>MEISETNIGIFYVSKLLALAPYSAKKNSKGQLEITRSWLFSIYSVCLCLIMVFLTYRGLLFDANSNIPVRMKSATSKVVTASDVSVVVLAIVTGVYCGMFGLRATQELNTRLDKIDSTLSPYNNVKKDRWRAYAMATVSLIVIGILLGLDVGTWVRMAQEMNISDEDTELNVQWYIPFYSLYFILTGLHINFANTAYGLGRRYKRLNQMLRTSYLSADKSYGNATNLVKVSTVKSISFKPMMPMALHASLTKLNTETLPNESATKNKSLLIRAMADNHESLGKCVRLLSRFYGIAVLFILVSCLLHLVATAYFLFLEMLNKRDNGYVWVQMLWIIFHFLRLLMVVEPCHLAAREARKTIQIVCEIERKVFEPILVEETKKFWQQLLVDDAEFSASGLCRVNRTILTSFASAIATYLVILIQFQKTNGLEGGSSGGWSHPQFEK[4x]

While mammals use G protein-coupled receptors (GPCRs) for sweet and bitter tastant perception, insects such as fruit flies use a unique family of proteins called gustatory receptors (Grs). To unravel the overall structure of these receptors and their unique structure features that define sugar specificity, we determined the cryo-electron microscopy (cryo-EM) structures of Drosophila mojavensis Gr43a (DmoGr43a) (given its better biochemical behavior than Drosophila melanogaster Gr43a (DmGr43a)) and Drosophila melanogaster Gr64a (DmGr64a) in apo or sugar-bound states. As expected, both DmoGr43a and DmGr64a form tetramer, and are topologically similar to each other, and to Orco from Apocrypta bakeri and odorant receptor 5 from Machilis hrabei (MhOR5)11. The structures of DmoGr43a and DmGr64a can be separated into a TMD with 28 transmembranes (TMs) in total (7 TMs in each subunit, numbered as S1–S7), and an intracellular domain (ICD) containing an “anchor domain”, following the nomenclature of Orco/MhOR510,11.

More recently, Gr43a and its homologs were identified as narrowly tuned fructose receptors, and they were also found to be expressed in the brain and function as a sensor for the hemolymph fructose levels, thereby regulating the feeding behaviors. Among different sugars tested, e.g., 100 mM maltose, arabinose, glucose, trehalose, and fructose, only fructose activated DmoGr43a, with a measured EC50 of 42.97 ± 4.69 mM and ~30 mM in electrophysiology and calcium imaging respectively. Lined by S7 that spans both ICD (S7a) and TMD (S7b), a continuous ion conduction pathway in the 4-fold symmetry axis runs all the way through both DmoGr43a and DmGr64a, and are all in the non-conductive state. In both proteins, two patches of constrictions are formed along the ion conduction pathway, one near the extracellular entrance (Ile 418 and Phe 422 for DmoGr43a, and Val 438 and Gln 441 for DmGr64a) and the other in the anchor domain in ICD (Leu 386 for DmoGr43a, and Glu 399 and Phe 403 for DmGr64a). Intriguingly, the narrowest point at the extracellular entrance is formed by completely different sets of residues in DmoGr43a and DmGr64a, e.g., bulky, hydrophobic phenylalanine in DmoGr43a vs smaller, hydrophilic glutamine in DmGr64a. Notably, Arg 70 from the S1–S2 loop, which is disordered in the apo state, becomes well-resolved in the fructose-bound state, and travels downward for fructose binding. When the apo and sugar-bound structures of DmoGr43a and DmGr64a were aligned, notable conformational changes could be revealed, mainly tilting of TM helices responsible for sugar binding towards bound sugars.1-(2-{[(3S)-3-(aminomethyl)-3,4-dihydroisoquinolin-2(1H)-yl]carbonyl}phenyl)-4-chloro-5-methyl-N,N-diphenyl-1H-pyrazole-3-carboxamide 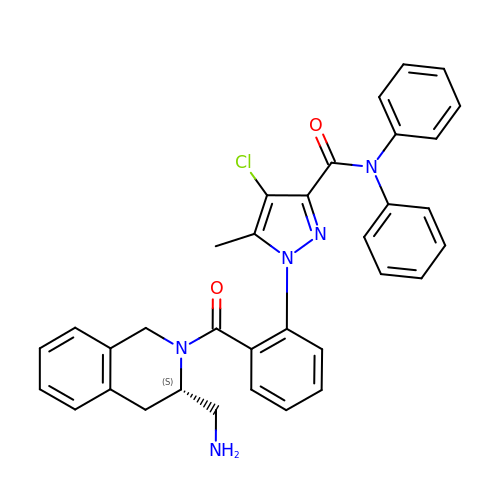| C34 H30 Cl N5 O2 | MLZCQGFPFQDFLC-NDEPHWFRSA-N>[2x]MAREELRRHLVGLIERSRVVIFSKSYCPHSTRVKELFSSLGVECNVLELDQVDDGA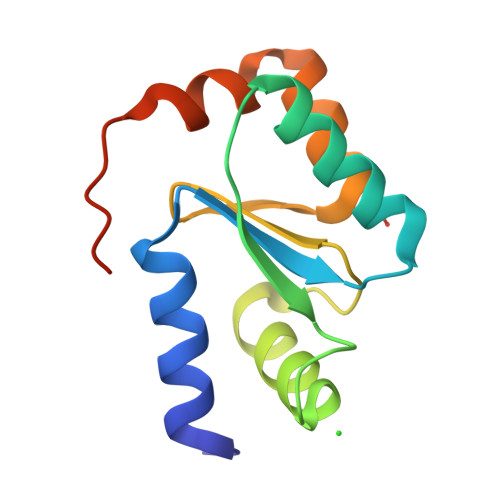RVQEVLSEITNQKTVPNIFVNKVHVGGCDQTFQAYQSGLLQKLLQEDLAYDAENLYFQ> GSHMRNVAAEQQLRELESTFDGRLGFVALDTATGARIAHRADERFPFCSTFKTMLSAAVLARSAGDAALLQRRIPYAKRDLVRYSPITEKHVGAGMTVAELCAATLQYSDNTAANLLIALLGGPQAVTAYARSIGDATFRLDRRETELNTAIPGDERDTTTIPGDERDTTTPAAMAASVRRLLVGDALGTAQRAQLNAWMLGNKTGDARIRAGVPAGWRVADKTGTGDYGTGNDIGVAYPPDRAPIVFVVYTTMRSRNAQARDDVIASAARIAARAFV

In class A β-lactamases, a conserved structural element called the omega loop5 constitutes a wall at the active site that shapes the binding cavity. PenL (NCBI reference sequence: YP_439646.1) is highly conserved in pathogenic Burkholderia species, including Burkholderia pseudomallei, Burkholderia mallei, and Burkholderia cenocepacia. PenL has been used as a model in exploring various evolutionary paths to substrate spectrum extension through amino acid substitutions, deletions, and duplications. In this study, we demonstrate the extensive perturbation-absorbing capacity of the omega loop against TR mutations of various sizes, some of which are large enough to include the entire omega loop.

CBA consists of two parts: a glycylboronate moiety that mimicks a transition state intermediate of acylation and a C7β side chain that mimicks the bulky C7β-aminothiazol carboxypropyloxyimino-amide side chain present in ceftazidime. The binding of CBA reduced the unmapped region by two residues, Ala171 and Ile172, in PenL-tTR10. More importantly, the α-helix of the omega loop was restored, consequently reestablishing the catalytic interactions among Glu166, Asn170, and the catalytic water W1. By contrast, the glycylboronate moiety of CBA exhibited a similar binding pattern in both PenL-tTRs, which mimicked the acylation transition state of β-lactam substrates and was similar to the bound conformation to other class A β-lactamases, such as TEM-1, CTX-M-9, and CTX-M-16634. In PenL-tTR10-CBA, the O12 of CBA was hydrogen-bonded to the Nδ2 of Asn132 and to W5, which was relocated to a position closer to Asn170. In addition, the thiazole ring of CBA had a ring-stacking interaction with the hydroxyphenyl ring of Tyr105. Although PenL-tTR10 and PenL-tTR11 exhibited differences from each other in their enzyme-ligand interaction patterns, their binding patterns were largely analogous to those in SHV-1 and CTX-M-9, respectively. It is of note that the B factors for CBA in PenL-tTR10-CBA (18.7 Å2) and PenL-tTR11-CBA (42.6 Å2) were higher than those in SHV-1 (16.1 Å2) and CTX-M-9 (10.9 Å2), respectively, suggesting more flexible active sites in the PenL-tTRs. Consistent with the structural data, the CD spectra of PenL-tTR10-CBA and PenL-tTR11-CBA showed that much of the altered profiles of the mutant enzymes were recovered upon CBA binding in the far-UV region (190~200 nm), reflecting induced-fit reformation of the active site. This recovery of the CD spectrum was more distinct with PenL-tTR10-CBA, which showed a highly-similar profile to that of PenL-WT. While PenL-tTR10 reconstituted the original conformation, PenL-tTR11 appeared to exploit the flexibility of the omega loop, allowing large conformational changes in the active site structure.>MTSCHIAEEHIQKVAIFGGTHGNELTGVFLVKHWLENGAEIQRTGLEVKPFITNPRAVKKCTRYIDCDLNRIFDLENLGKKMSEDLPYEVRRAQEINHLFGPKDSEDSYDIIFDLHNTTSNMGCTLILEDSRNNFLIQMFHYIKTSLAPLPCY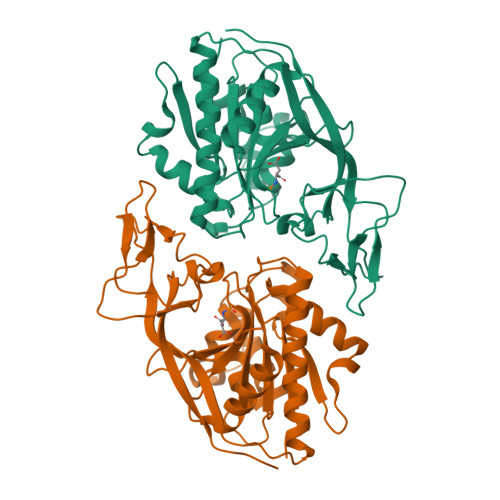VYLIEHPSLKYATTRSIAKYPVGIEVGPQPQGVLRADILDQMRKMIKHALDFIHHFNEGKEFPPCAIEVYKIIEKVDYPRDENGEIAAIIHPNLQDQDWKPLHPGDPMFLTLDGKTIPLGGDCTVYPVFVNEAAYYEKKEAFAKTTKLTLNAKSIRCCLH[2x]> 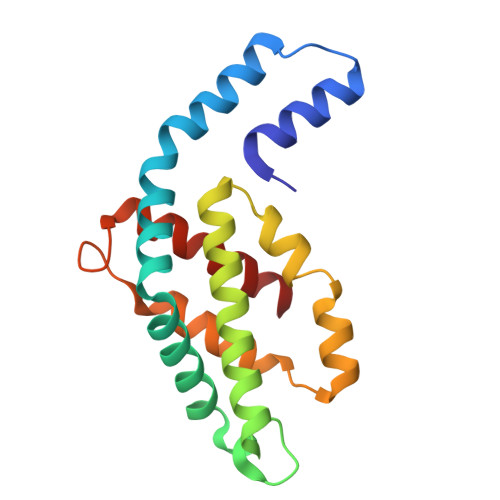MKSVVTTVIAAADAAGRFPSSSDLESVQGSIQRSAARLEAAEKLAGNIDAVAQEAYNACIQKYPYLNNSGEANSTDTFKAKCLRDVKHYMRLIQYSLVVGGTGPLDEWGIAGQREVYRALGLPTAPYVEALSFARNRGCAPRDMSAQALTEYNALLDYAINSLS> GMAGAAHRLMEARMRRYDNKF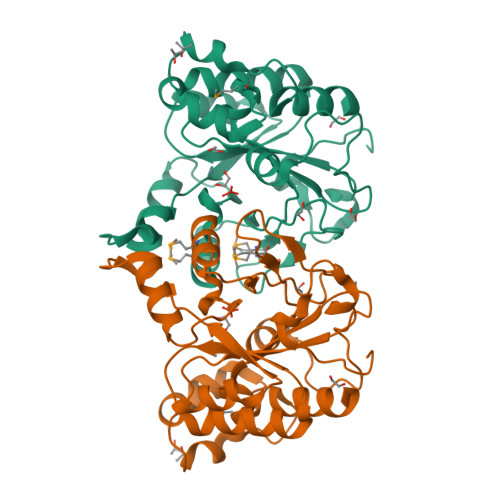ARISDIDINQPESWRGRIFLTFDIDWAADFVLQDTIDLIEGAGVCATWFATHSTPLLENIRRNPLFELGVHPNFNPLLAGAHAEGVQEILDRTLELAPGCVSVRSHSLVQATSILNMFGERRLRYDCNILVPWDAGIVLQPWRHWTGDMVRVPYLWEDDVACLYDWEFDSTFDYWYQPDGINVLDFHPIHVYMNTESLRRYEDSREVHRNPVDLIRWRNTSAGSRTFLQSLLARNI>[4x]MLNSFKLSLQYILPKLWLTRLAGWGASKRAGWLTKLVIDLFVKYYKVDMKEAQKPDTASYRTFNEFFVRPLRDEVRPIDTDPNVLVMPADGVISQLGKIEEDKILQAKGHNYSLEALLAGNYLMADLFRNGTFVTTYLSPRDYHRVHMPCNGILREMIYVPGDLFSVNHLTAQ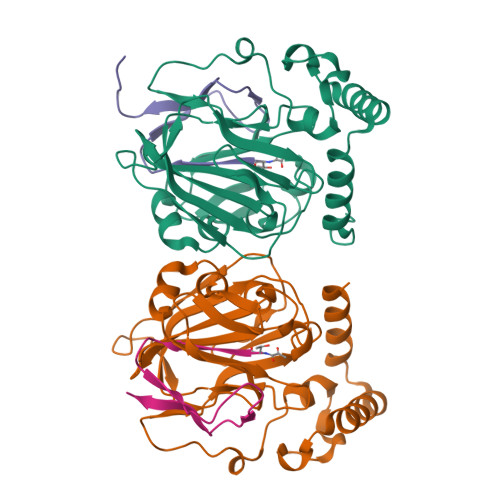NVPNLFARNERVICLFDTEFGPMAQILVGATIVGSIETVWAGTITPPREGIIKRWTWPAGENDGSVALLKGQEMGRFKLG;>[4x]XTVINLFAPGKVNLVEQLESLSVTKIGQPLAVSTGHHHHHHG>GSHMDRISVPPLNTKRLLPTRYKTKNAIMSILRNGEVVLEFLKFRPTYNEDRINDICRI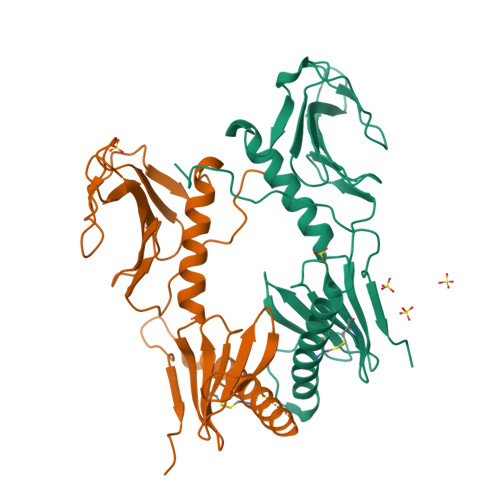SDDGQRIIIYQPDPGRGLPVREQPPDLQIPSGDCVYNYDNLPSKHWKKYIYGARFVGLVKSKTPKVTYFSTLGKCQLMETMTDFEIRFYSGAKLLKTPSEGLKVYDRNGMLLSDYSCSESRSLIEHGNECFTHCVNISNALEVAQTKDNSCFPVTIGRRPITDVQP[2x]>[2x]KTEMKDDFAKLEEQFDAKLGIFALDTGTNRTVTYRPDERFAFASTIKALTVGVLLQQKSIEDLNQRITYTRDDLVNYNPITEKHVDTGMTLKELADASLRYSDNTAQNLILKQIGGPESLKKELRKIGDEVT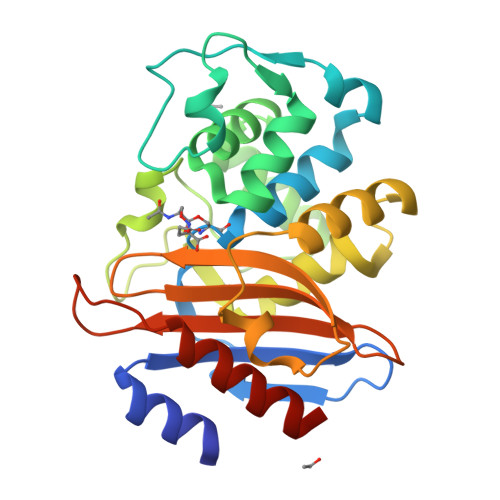NPERFEPELNEVNPGETQDTSTARALATSLQAFALEDKLPSEKRELLIDWMKRNTTGDALIRAGVPEGWEVADKTGAGSYGTRNDIAIIWPPKGDPVVLAVLSSRDKKDAKYDDKLIAEATKVVVKALNMNGK> LSYFQALPLAQRVSIMVALPFVYTITWQLLYSLRKDRPPLVFYWIPWVGSAIPYGTKPYEFFEDCQKKYGDIFSFMLLGRIMTVYLGPKGHEFIFNAKLADVSAEAAYSHLTTPVFGKGVIYDCPNHRLMEQKKFVKGALTKEA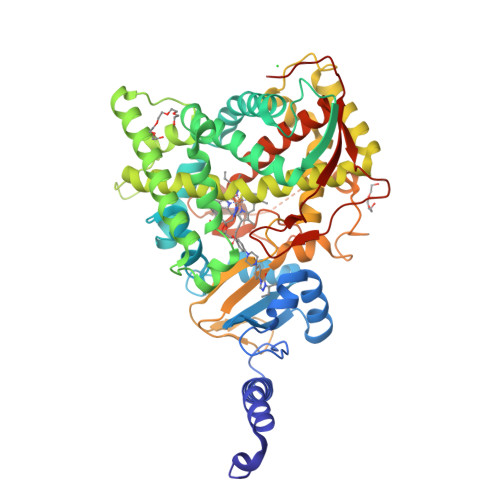FVRYVPLIAEEIYKYFRNSKNFKINENNSGIVDVMVSQPEMTIFTASRSLLGKEMRDKLDTDFAYLYSDLDKGFTPINFVFPNLPLEHYRKRDHAQQAISGTYMSLIKERREKNDIQNRDLIDELMKNSTYKDGTKMTDQEIANLLIGVLMGGQHTSAATSAWCLLHLAERPDVQEELYQEQMRVLNNDTKELTYDDLQNMPLLNQMIKETLRLHHPLHSLFRKVMRDVAIPNTSYVVPRDYHVLVSPGYTHLQEEFFPKPNEFNIHRWDGDAASSSAAGGDEVDYGFGAISKGVSSPYLPFGGGRHRCIGELFAYCQLGVLMSIFIRTMKWRYPTEGETVPPSDFTSMVTLPTAPAKIYWEKRHPEQKYG>[2x]PSVYDAAAQLTADVKKDLRDSWKVWGSDKKGNGVALMTTLFADNQETIGY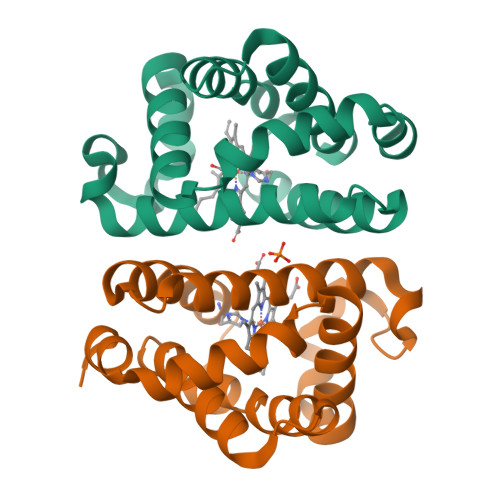FKRLGDVSQGMANDKLRGHSITLMYALQNFIDQLDNPDDLVCVVEKFAVNHITRKISAAEFGKINGPIKKVLASKNFGDKYANAWAKLVAVVQAAL>[2x]GMTNVELVFIPSPGLSHLVSTVEAAKLLLHRDHRLSITVLITNLHKDTKVENYTLKTTSNPNTSPRLRFINLPTQEEDS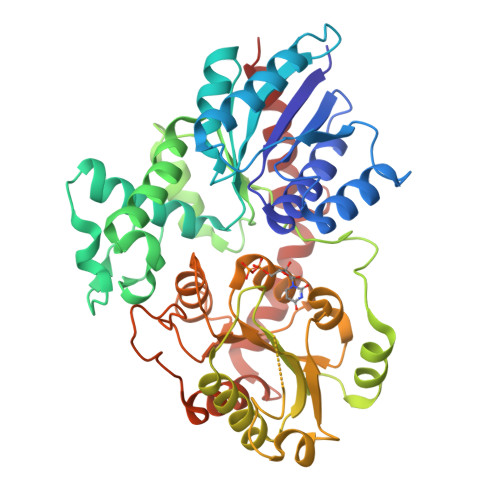IDSQIRQVREIVSVLIKNPDSKLGGLVLDMFCTSFIQVAEEFAIPSYVFFTSGASALGLLQHLVSLKLEHNQDLTQFKDSDVELSVPCFSVPVPAKVLPAVMVEGGPIEDTFMNYFKRIPETRGIMVNTFYELESFAIQSLLSDAKAPKVYPVGPILGFDQTQGPVGDDAIKKWLDDQPENSVVFLCFGTMGSFCEGQVKEIAMALEKSGNRFLWSLRKPEKGRVTEYENYEEVLPQGFLERTKGVGKVMGWAPQAAVLSHPAVGGFVSHCGWNSTLESLWFGVPMATFPLYAEQQMNAFLLVKEEGMAEMITLDYKIDFKGEKQPEIVGSDEIEAAIRRLMAEESGVRRKVKEMQNKARSALLEGGSSYDAQCLFVHDVINNIG> GVPTYLLPG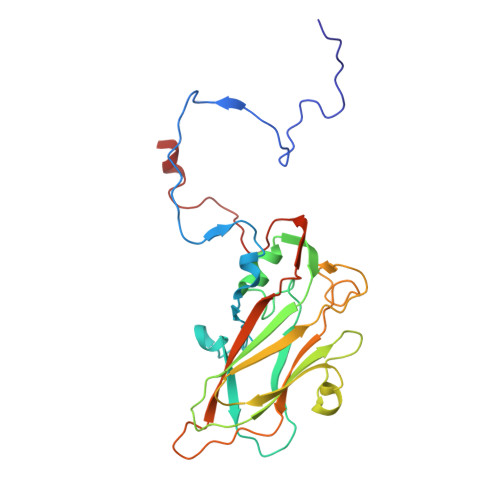SGQFLTTDDHSSAPVLPCFNPTPEMHIPGQVRNMLEVVQVESMMEINNTESAVGMERLKVDISALTDVDQLLFNIPLDIQLDGPLRNTLVGNISRYYTHWSGSLEMTFMFCGSFMATGKLILCYTPPGGSCPTTRETAMLGTHIVWDFGLQSSVTLIIPWISGSHYRMFNNDAKSTNANVGYVTCFMQTNLIVPSESSDTCSLIGFIAAKDDFSLRLMRDSPDIGQIDHLHAAEAAYQ>MSEKDEYQFQHQGAVELLVFNFLLILTILTIWLFKNHRFRFLHETGGAMVYGLIMGLILRYATAPTDIESGTVYDCGKLAFSPSTLLINITDQVYEYKYKREISQHNINPHLGNAILEKMTFDPEIFFNVLCPPIIFHAGYSLKKRHFFQNLGSILTYAFLGTAISCIVIGLIMYGFVKAMVYAGQLKNGDFHFTDCLFFGSLMSATDPVTVLAIFHELHVDPDLYTLLFGESVLNDAVAIVLTYSISIYSPKENPNAFDAAAFFQSVGNFLGIFAGSFAMGSAYAVVTALLTKFTKLCEFPMLETGLFFLLSWSAFLSAEAAGLTGIVAVLFCGVTQAHYTYNNLSLDSKMRTKQLFEFMNFLAENVIFCYMGLALFTFQNHIFNALFILGAFLAIFVARACNIYPLSFLLNLGRKHKIPWNFQHMMMFSGLRGACAFALAIRDTESQPKQMMFSTTLLLVFFTVWVFGGGTTPMLTWLQIRVGVDLDEDLKERPSSHQEANNLEKSTTKTESAWLFRMWYGFDHKYLKPILTHSGPPLTTTLPEWCGPISRLLTSPQAYGEQLKEGENLYFQ[2x]

Na+/H+ exchangers facilitate the exchange of monovalent cations (Na+/Li+/K+) and protons (H+) across membranes to regulate intracellular pH, sodium levels and cell volume. Na+/H+ exchangers that perform this task are physiological homodimers, and whilst the ion transporting domain is highly conserved, their dimerization differs. The transporter is made up of two distinct domains, a dimerization domain and an ion-transporting (core) domain. Here, we report cryo-EM structures of E. coli NhaA and E. caballus NHE9 in complex with cardiolipin and phosphatidylinositol-3,5-bisphosphate PI(3,5)P2 lipids binding at their respective dimer interfaces.

To improve the resolution of the NHE9* structure we substituted L139 and I444 residues to cysteines in an attempt to disulphide-trap the inward-facing state. We subsequently collected a larger data-set of 13,780 movies and the final 3D-reconstruction had 78,370 particles from which an EM map was reconstructed to 3.2 Å according to the gold-standard Fourier shell correlation (FSC) 0.143 criterion. Map density and sulphur atom distances, however, did not support disulphide bond formation between the two introduced cysteine residues. Given that NHE9* co-purified from yeast with several lipids corresponding to the molecular mass of PIP224, we attempted to model two PIP2 lipids into the NHE9* CC maps and found that the density was a better fit for the phosphatidylinositol-3,5-bisphosphate PI(3,5)P2, lipid, rather than the more abundant phosphatidylinositol-4,5-bisphosphate PI(4,5)P2 lipid. The glycerol backbone and acyl chains of the PI(3,5)P2 lipid form hydrophobic stacking interactions to W321 (TM8, TM8’). Two glutamine residue Q17 (TM1, TM1’) and N136 (TM3, TM3’) are well positioned to hydrogen-bond with the C3-phosphate group. The position of these polar residues could partially explain the preference for PI(3,5)P2 lipids, since there are no polar residues close enough to interact with a phosphate group at the C4-OH position. Following a rigid-body fit of the TM2-TM3 β-hairpin loop domain in the NHE9*CC maps, the positively-charged loop domain residues K105, K105’ K107, K107’ were aligned to help neutralize the negatively-charge headgroups of PI(3,5)P2. In the improved NHE9*CC structure, we could model part of the C-terminal tail without protein complex partners. However, in the absence of a regulatory protein, the C-terminal interfacial helix in NHE9*CC is making a number of direct contacts with the linker helix TM7 through interaction with a lysine residue, likely restricting its mobility and that of the core transport domains.> GAMANAVIGNVVTRFPPEPSGYLHVGHAKAAFLNNYYAQMYEGKMLLRFDDTNPVLEDIKYEKSIIEDLENLGLKYEKISYSSDHFDLLEKYCIDMIKMNKAYADDTGVEDMRNQRGEGIESINRNNSIEKNLELFNEMRKGTEIGQKNCIRAKINMQSKNKCMRDPVMYRCIVDVPHHKHQFKYKCYPTYDFACPIIDSIEGVTHALRTNEYSDRIEQYNWFISTLNLRKVYIYEFSRLAFVKTVMSKRKLKWFVENNVVDSWVDPRFPT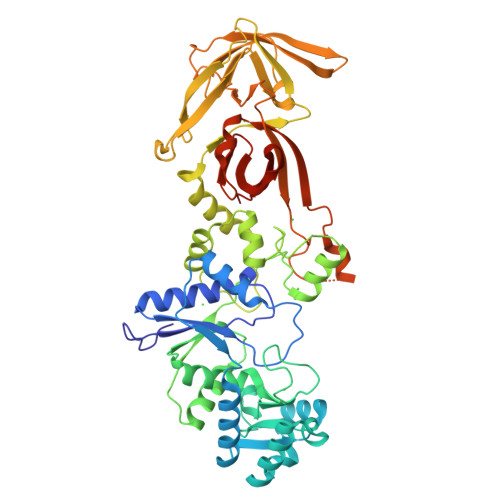IKGILRRGLTKEALFQFILEQGPSKAGNLMQWDKLWSINKQIIDPIIPRYAAVDKNSSILLILTDLTDQVIQKERDLHMKNKSLGTCNMYYNNKYLIELEDAQTLLENEEITLIKLGNIIIKNIEKENGKIKQINALSNFHGDFKTTKKKIHWLPYLPQQLITCTLYEYDHLITVDKFENDNKDDWTNFINFNSKHETLVYAEPSISSLKVSDKFQFERRGYFILDKIDPHHHLHLIKIPDGKSKNMSIITT>[2x]QQYVNINPPMPSDTPGKIEVLEFFAYTCPHCAAIEPMVEDWAKTAPQDVVLKQVPIAFNAGMKPLQQLYYTLQALERPDLHPKVFTAIHTERKRLFDKKAMGEWAASQGVDRAKFDSVFDS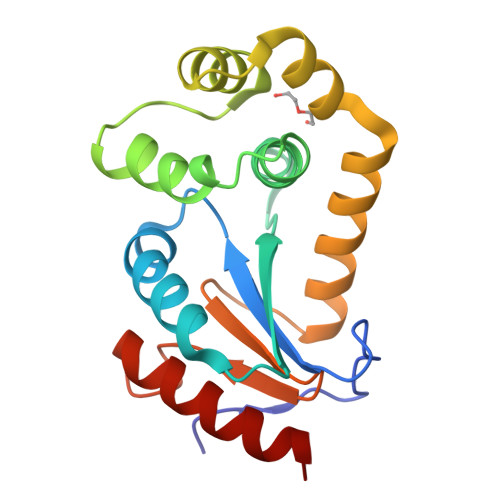FSVQTQVQHASQLAEAAHIDGTPAFAVGGRYMTSPVLAGNDYAGALKVVDQLIVQSRK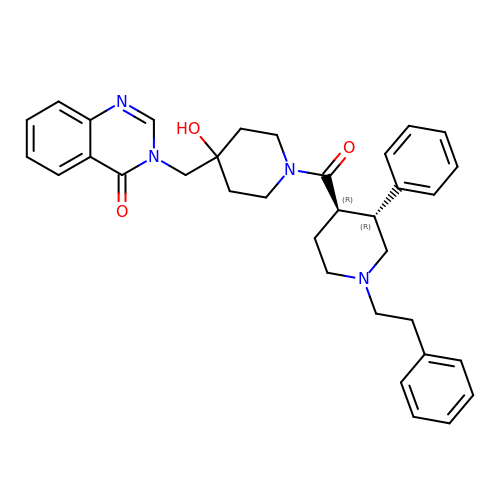3-[[4-oxidanyl-1-[(3~{R},4~{R})-3-phenyl-1-(2-phenylethyl)piperidin-4-yl]carbonyl-piperidin-4-yl]methyl]quinazolin-4-one | C34 H38 N4 O3 | RLVSZASCPMMLKY-DGPALRBDSA-N> GEDSLGMEVGYRLIPMVDFQQDGELLGRIRSIRKKFAQDMGFLPPVVHIRDNMDLQPARYRILMKGVEIGSGDAYPGRWLAINPGTAAGTLPGEKTVDPAFGLDAIWIESALKEQAQIQGFTVVEASTVVATHLNHLIGQFSAELFGRQEAQQLLDRVSQEMPKLTEDLVPGVVTLTTLHKVLQNLLAEKVPIRDMRTILETLAEHAPLQSDPHELTAVVRVALGRAITQQWFPGNEEVQVIGLDTALERLLLQALQGGGGLEPGLADRLLAQTQEALSRQEMLGAPPVL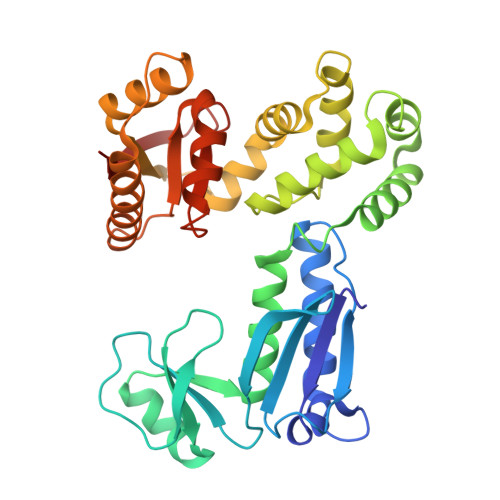LVNHALRPLLSRFLRRSLPQLVVLSNLELSDNRHIRMTATIGGK>[6x]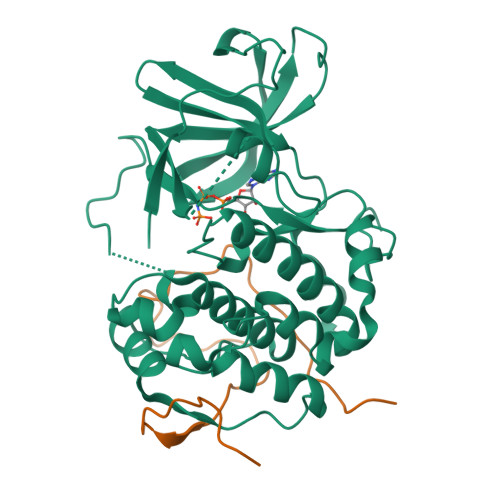GSASNPQTEEVSIKEIAITHHVKEGHEKADPSQFELLKVLGQGSFGKVFLVKKISGSDARQLYAMKVLKKATLKVRDRVRTKMERDILVEVNHPFIVKLHYAFQTEGKLYLILDFLRGGDLFTRLSKEVMFTEEDVKFYLAELALALDHLHSLGIIYRDLKPENILLDEEGHIKLTDFGLSKESIDHEKKAYSFCGTVEYMAPEVVNRRGHTQSADWWSFGVLMFEMLTGTLPFQGKDRKETMTMILKAKLGMPQFLSPEAQSLLRMLFKRNPANRLGAGPDGVEEIKRHSFFSTIDWNKLYRREIHPPFKPATGRP;>GSRMLPIEGAPRRRPPVKFIFPPPPLSSLPGFGRPRGYAGPTVIDMSAPDDVFAEDTPSPPAT[6x]>[14x]MALVPVVVEQTGRGERSYDIFSRLLKDRIIFLGDQVNDATAGLIVAQLLFLEAEDPDKDIHL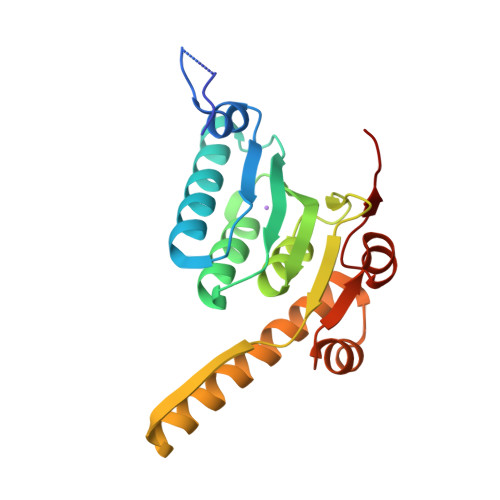YINSPGGSITSGMAIYDTMQYIKPDVSTICIGMAASMGAFLLAAGAKGKRLALPNSEIMIHQPLGGAQGQATDIEIHAKRILKIKETLNEILSERTGQPLEKIKMDTERDNFMSALEAKEYGLIDEVFTKRP>[5x]MITKSNEFWTPKRLLETDDRIFLVVGGRGVGKTFNVTGE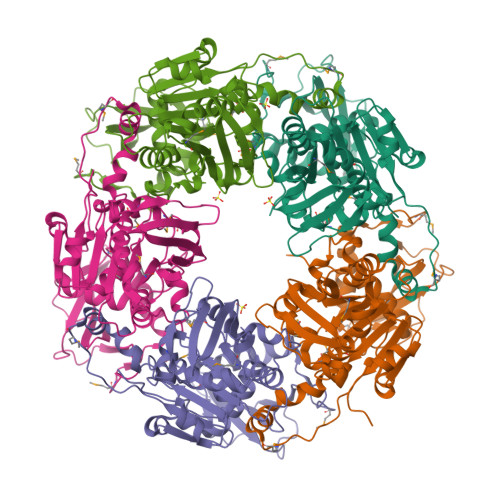ALDDLFFNNVSMVYLRRLGVEIDELEKNNFITEEMLRVYFGNRFSDFNADESKQIMRFSIDGAIHEIKAIRNKIFFDDRCIVYFIALSRAGHVKSNNYPDVKYLVFDEVIIDRSIMPNARYIRNEFTVLLNLIETIKRKREDFYLFMLSNVGENFNPIFAGLGYYLTHEDIKKGFVKREDYCVQFVENKQEELNMTDPFVRLGAKNRDFSNSKTNAFENIRTPYFKHYGKKPKLLVKYDRQYLGIAERKIPSGLEYYYQVYKTLDGLENITVFNNNFDTLMEDEVFLEETQLKKKFKTYFELFQQNMVYHESPETFLEWSKFVYALKLEHHHHHH> GPIIVEPHVTAVWGKNVSLKCL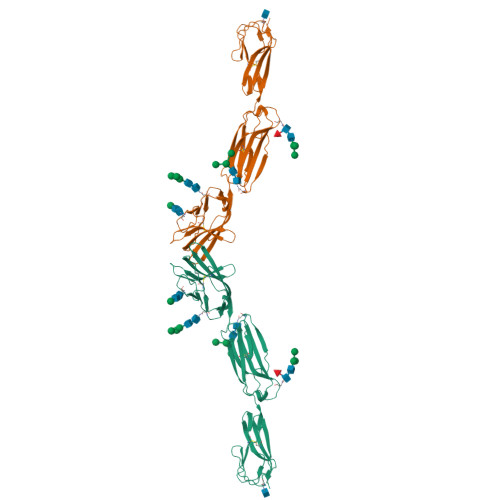IEVNETITQISWEKIHGKSSQTVAVHHPQYGFSVQGEYQGRVLFKNYSLNDATITLHNIGFSDSGKYICKAVTFPLGNAQSSTTVTVLVEPTVSLIKGPDSLIDGGNETVAAICIAATGKPVAHIDWEGDLGEMESTTTSFPNETATIISQYKLFPTRFARGRRITCVVKHPALEKDIRYSFILDIQYAPEVSVTGYDGNWFVGRKGVNLKCNADANPPPFKSVWSRLDGQWPDGLLASDNTLHFVHPLTFNYSGVYICKVTNSLGQRSDQKVIYISDPPHHHHHH>[6x]SGSEPTKVMVAVNASTIKDYPNPSISCKRAFEWT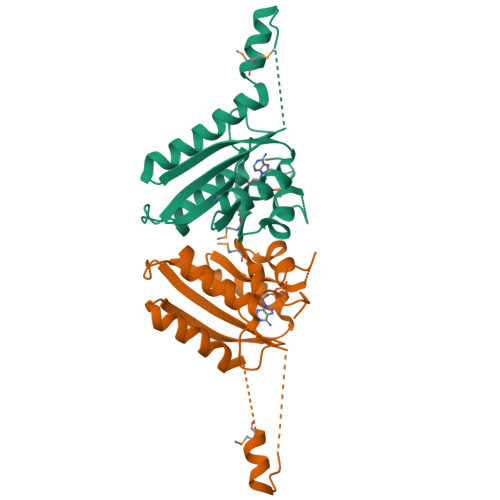LEKIVRSNTSDFKILLLHVQVVDEDGFDDVDSIYASPEDFRDMRQSNKAKGLHLLEFFVNKCHEIGVGCEAWIKTGDPKDVICQEVKRVRPDFLVVGSRGLGRFQKVFVGTVSAFCVKHAECPVMTIKRNADETPSDPADD>DLADRFAELERRYDARLGVYVPATGTTAAIEYRADERFAFCSTFKAPLV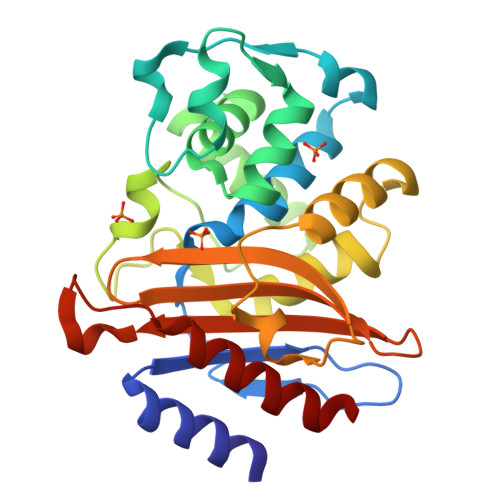AAVLHQNPLTHLDKLITYTSDDIRSISPVAQQHVQTGMTIGQLCDAAIRYSDGTAANLLLADLGGPGGGTAAFTGYLRSLGDTVSRLDAEAPELNRDPPGDERDTTTPHAIALVLQQLVLGNALPPDKRALLTDWMARNTTGAKRIRAGFPADWKVIDKTGTGDYGRANDIAVVWSPTGVPYVVAVMSDRAGGGYDAEPREALLAEAATCVAGVLA[4x]The effector RidL binds the Vps29 retromer subunit, blocks retrograde vesicle trafficking, and promotes intracellular bacterial replication. The 131-kDa Icm/Dot substrate RidL binds the retromer subunit Vps29 as well as PtdIns(3)P and impairs retrograde trafficking. Here, we show that the 29-kDa N-terminal domain of RidL (RidL2–281) adopts a “foot-like” fold comprising a protruding hydrophobic β-hairpin, which determines the interaction with the Vps29 retromer subunit and displaces the regulator TBC1D5 from the retromer. Thus, the hydrophobic β-hairpin of RidL is critical for binding of the L. pneumophila effector to the Vps29 retromer subunit and displacement of the regulator TBC1D5.

Using this approach, we obtained well-diffracting crystals of the N-terminal 29 kDa fragment (aa 2–281) belonging to space group I422 with one molecule in the asymmetric unit. The structure of RidL2–281 was solved at 1.9-Å resolution. The electron densities allowed for building a model comprising residues 7–274. The structure features a “foot-like” fold, consisting primarily of interacting bundles of α-helices connected by loops of various lengths. The surface representation of B-factors indicates an increasing flexibility from the heel to the toes of the foot. At the heel of the foot, positioned between helices 8 and 9, there is a surface-exposed hairpin formed by 2 antiparallel β-strands connected by a loop comprising 5 residues (aa 160–180, termed “β-hairpin”). The β-hairpin is structurally well defined and rigid, as well as hydrophobic (based on surface charge distribution). The β-hairpin and in particular the sequence motif PTIPP at its tip is conserved among L. pneumophila RidL homologs. The three prolines in this motif break the antiparallel β-strands and stiffen the tip of the loop. Thereby, the side chain of the conserved Ile170 forms an exposed hydrophobic spot.

> GPSILEEYIRMAKNKEFFDALEEIAESAKNDETLRNELAKVLDDILKTDPSDPEAFRKIVAEHQEFWDEHDPSLMEFNEGRFFGKSRKQYLKSDDFLNSTDPTYNFQKLHQFAAEQRVKLGLEKSDTDTLVAILKNNPEECRAYIESKKPGLGNFSEGNVHGWLKEEYTPTIPPKAINKSTGVLSDEAIKRIKEQARDLLLLKLINSSGNTQLLKDLRDAMSKPEAERAANALGFPTEGNGVLFLSREVVDALEERVEKLEQEAAKRGFDSYVQSLSHNALLA> KEFTLDFSTAKTYVDSLNVIRSAIGTPLQTISSGGTSLLMIDSGTGDNLFAVDVRGIDPEEGRFNNLRLIVERNNLYVTGFVNRTNNVFYRFADFSHVTFPGTTAVTLSGDSSYTTLQRVAGISRTGMQ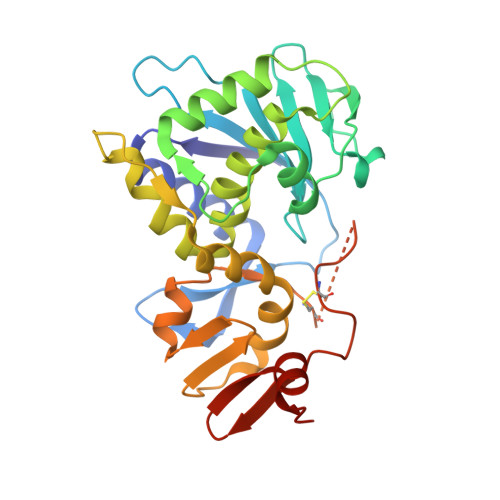INRHSLTTSYLDLMSHSGTSLTQSVARAMLRFVTVTAEALRFRQIQRGFRTTLDDLSGRSYVMTAEDVDLTLNWGRLSSVLPDYHGQDSVRVGRISFGSINAILGSVALILNCHHHASRVARMASDEFPSMCPADGRVRGITHNKILWDSSTLGAILMRRTISS> MDHDFLKGQGDARSVRHIAIPAHRGLITDRNGEPLAVSTPVTTLWANPKELMTAKERWPQLAAALGQDTKLFADRIEQNAEREFIYLVRGLTPEQGEGVIALKVPGVYSIEEFRRFYPAGEVVAHAVGFTDVDDRGREGIELAFDEWLAGVPGKRQVLKDRRGRVIKDVQVTKNAKPGKTLALSIDLRLQYLAHRELRNALLENGAKAGSLVIMDVKTGEILAMTNQPTYNPNNRRNLQ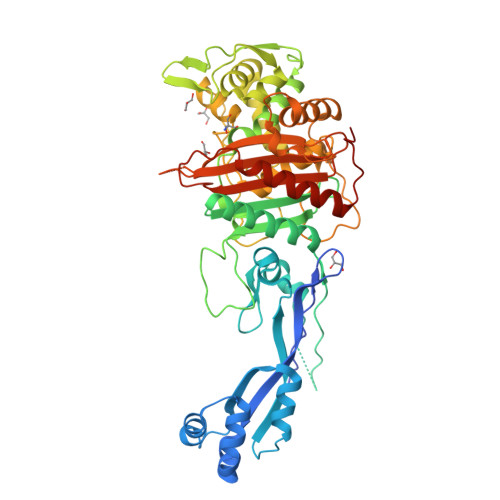PAAMRNRAMIDVFEPGSTVKPFSMSAALASGRWKPSDIVDVYPGTLQIGRYTIRDVSRNSRQLDLTGILIKSSNVGISKIAFDIGAESIYSVMQQVGLGQDTGLGFPGERVGNLPNHRKWPKAETATLAYGYGLSVTAIQLAHAYAALANDGKSVPLSMTRVDRVPDGVQVISPEVASTVQGMLQQVVEAQGGVFRAQVPGYHAAGKSGTARKVSVGTKGYRENAYRSLFAGFAPATDPRIAMVVVIDEPSKAGYFGGLVSAPVFSKVMAGALRLMNVPPDNLPTAKLVPRG> VPDSIDYRKKGYVTPVKNQGQCGSCWAFSSAGALEGQLKKKTGKLLALSPQNLVDCVTENYGCGGGYMTTAFQYVQQNGGIDSEDAYPYVGQDESCMYNATAKAAKCRGYREIP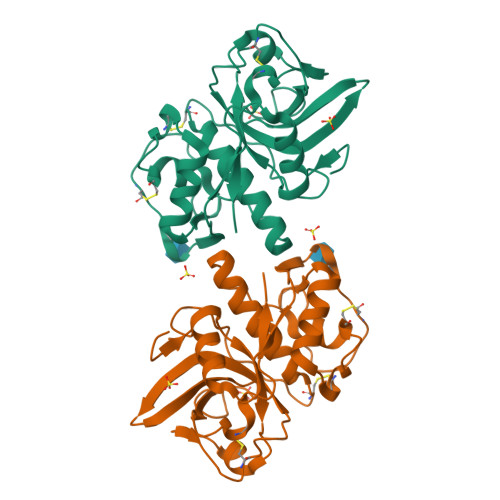VGNEKALKRAVARVGPISVSIDASLASFQFYSRGVYYDENCDRDNVNHAVLVVGYGTQKGSKHWIIKNSWGESWGNKGYALLARNKNNACGITNMASFPKM> MSRLDKSKVINSALELLNEVGIEGLTTRKLAQKLGVEQPTLYWHVKNKRALLDALAIEMLDRHHTHFSPLEGESWQDFLRNNAKSFRNALLSHRDGAKVHLGTRPTEKQYETLENQLAFLTQQGFSLENALYALSAVGHFTLGSVLEDQEHQVAKEERETPTTDSMPPLLRQAIELFDHQGAEPAFLHGLESLIRGFEVQLTALLQIV;> KKESRVVVW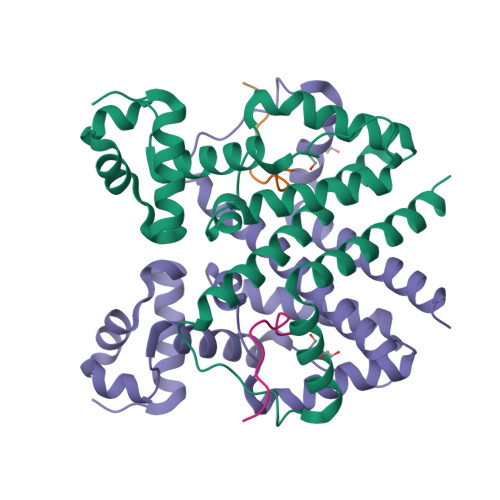RLPPLH4-[(3-{2-[(2-methoxyethyl)amino]-2-oxoethyl}-1,3-benzothiazol-3-ium-2-yl)methyl]-1-methylquinolin-1-ium 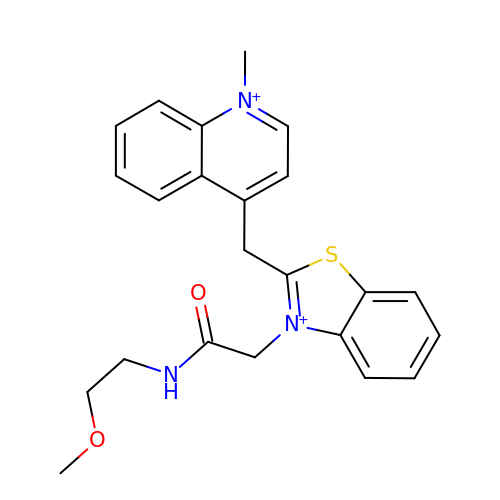| C23 H25 N3 O2 S | WEFGJTSJMBBARG-UHFFFAOYSA-O>PPYTVVYFPVRGRCAALRMLLADQGQSWKEEVVTVETWQEGSLKASCLYGQLPKFQDGDLTLYQSNTILRHLGRTLGLYGKDQQEAALVDMVNDGVEDLRCKYASLIYTNYEAGKDDYVKALPGQLKPFETL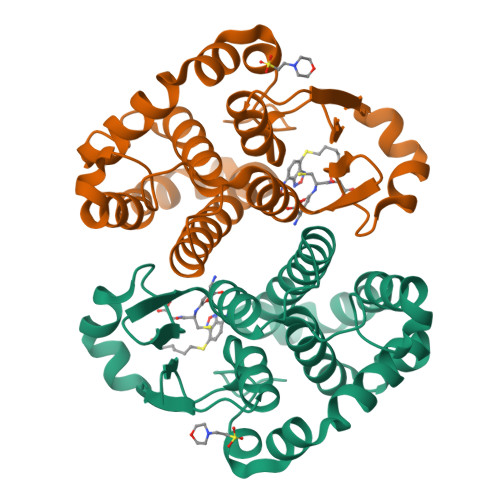LSQNQGGKTFIVGDQISFADYNLLDLLLIHEVLAPGCLDAFPLLSAYVGRLSARPKLKAFLASPEYVNLPINGNGKQ[2x]>MDIKELHVKTVKRGENVTMECSMSKVTNKNNLAWYRQSFGKVPQYFVRYYSSNSGYKFAEGFKDSRFSMTVNDQKFDLN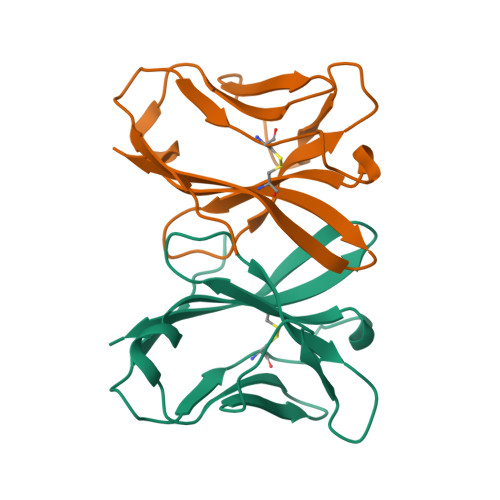IIGAREDDGGEYFCGEVEGIIIKFTSGTRLQF[4x]>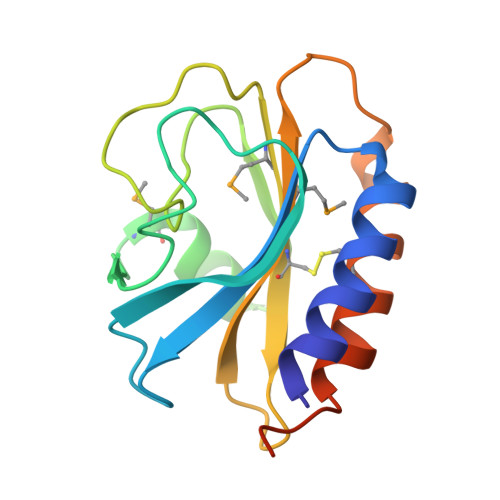 RFESVALEQLQIVHISSEADFSAVYSFRPKNLNYFVDIIAYEGKLPSTISEKSLGGYPVDKTMDEYTVHLNGRHYYSNSKFAFLPTKKPTPEINYMYSCPYFNLDNIYAGTITMYWYRNDHISNDRLESICAQAARILGRAKKLAAALEHHHHHH>[8x]MAEKPKLHYFNGRGRMESTRWLLAAAGVEFEEKFIKSAEDLDKLRNDGYLMFQQVPMVEIDGMKLVQTRAILNYIA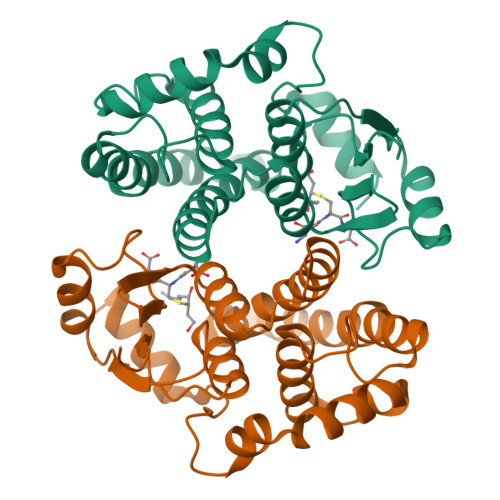SKYNLYGKDIKERALIDMYIEGIADLGEMIIMLPFCPPEEKDAKLALIKEKIKNRYFPAFEKVLKSHGQDYLVGNKLSRADIHLVELLYYVEELDSSLISSFPLLKALKTRISNLPTVKKFLQPGSPRKPPPDEIYVRTVYNIFRP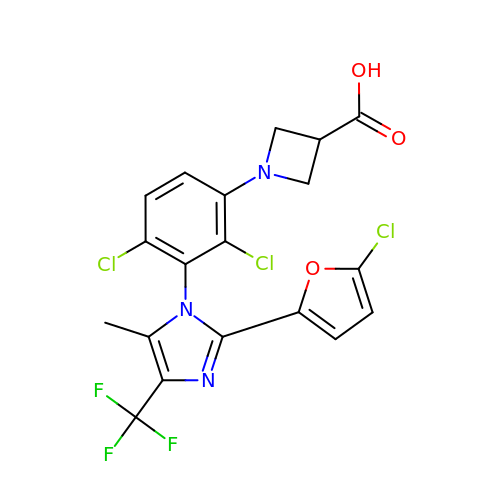1-[2,4-bis(chloranyl)-3-[2-(5-chloranylfuran-2-yl)-5-methyl-4-(trifluoromethyl)imidazol-1-yl]phenyl]azetidine-3-carboxylic acid | C19 H13 Cl3 F3 N3 O3 | XHCGKVYORHHKEM-UHFFFAOYSA-N>[6x]IPGANLLRMAFGVIGTQIVRYRKFEQRVKNDQAQYVSMFGEPFDLAASVQRVRRDQYAQFNLEFQRNYVMIFANFDMVDLDRNMAGDQFLWTGRVFQLESQGSWFYQDGWGVCLAVDIGAAKA;>[12x]MVIFDEHKFRTLFPEFADPAAYPDVRLQMYFDIACEFISDRDSPYRILNGKALEACLYLLTAHLLSLSTMQVQGAAGGGVTAGGTQGGFITSATVGEVSVAKLAPPAKNGWQWWLSGTPYGQELWALLSVKAVGGFYIGGLPERRGFRKVGGTFW;>[6x]MFDGELIAKLVVELNAAMTSAQEALQFPDFEVVQKAQPTQQGTSTRPTIFFQKLFDIPRGWPATDWHLDNTARKYVEITRQHVETTFQISSLHWQNPEITHVVTASDIANYVRAYFQARSTIERVKELDFLILRVSQISNEAFENDNHQFEFHPSFDMVVTYNQYIRL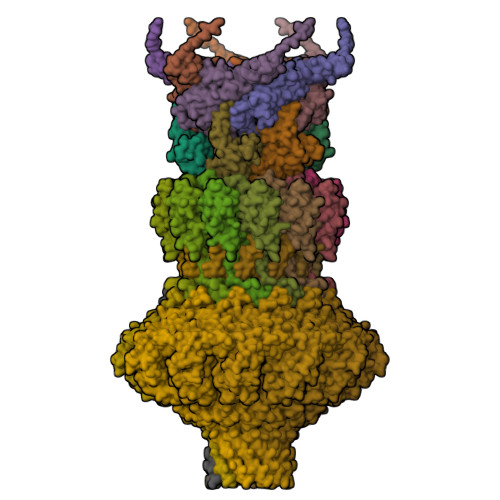YENAAYSADGVLIG;>[12x]PTMLQDWYNSQGFIGYQACAIISQHWLVDKACSMSGEDAARNGWELKSDGRKLSDEQSALIARRDMEFRVKDNLVELNRFKNVFGVRIALFVVESDDPDYYEKPFNPDGVTPGSYKGISQIDPYWAMPQLTAGSTADPSSEHFYEPDFWIISGKKYHRSHLVVVRGPQPPDILKPTYIFGGIPLTQRIYERVYAAERTANEAPLLAMSKRTSTIHVDVEKAIANEEAFNARLAFWIANRDNHGVKVLGIDEGMEQFDTNLADFDSIIMNQYQLVAAIAKTPATKLLGTSPKGFNATGEHETISYHEELESIQEHIFDPLLERHYLLLAKSEEIDVQLEIVWNPVDSTSSQQQAELNNKKAATDEIYINSGVVSPDEVRERLRDDPRSGYNRLTDDQAETEPGMSPENLAEFEKAGAQSAKAKGEAERAEAQAG>CTAITYVSKDHYFGRNFDYEISYNEVVTITPRNYKFSFREVGNLDHHFAIIGIAAGIADYPLYYDAINEKGLGMAGLNFSGYADYKKIEEGKENVSPFEFI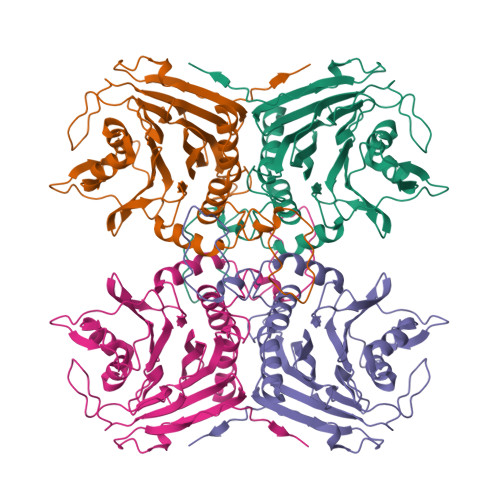PWVLGQCSTVDEAKKLLKNLNLVNINFSDELPLSPLHWLLADKEQSIVVESTKEGLRVFDNPVGVLTNNPTFDYQLFNLNNYRVLSTRTPKNNFSDQIELDIYSAGMGGIGLPGDLSSVSRFVKATFTKLNSVSRSSEYESISQFFHILSSVEQQKGLCDVGDEKYEYTIYSSCCNLEKGIYYYRTYDNSQITAVDMNKENLEKDSLIVYPMVETQQINYANLEHHHHHH[4x]>SNAMIITIPIKNQKDIGTPSDSVVVLGYFDGIHKGHQELFRVANKAARKDLLPIVVMTFNESPKIALEPYHPDLFLHILNPAERERKLKREGVEELYLLDFSSQFASLTAQEFFATYIKAMNAKIIVAGFDYTFGSDKKTAEDLKNYFDGEVIIVPPVEDEKGKISSTRIRQAILDGNVKEAGKLLGAPLPSRGMVVHGNARGRTIGYPTANLVLLDRTYMPADGVYVVDVEIQRQKYRAMASVGKNV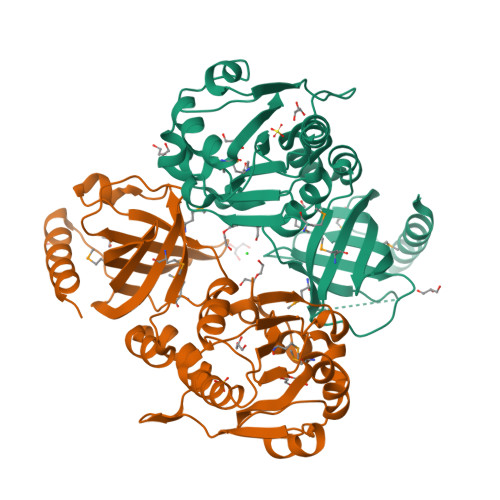TFDGEEARFEVNIFDFNQDIYGETVMVYWLDRIRDMTKFDSVDQLVDQLKADEEVTRNWS[3x]> MFYIDNDSGVTVMPPVSAQRSAIVRWFSEGDGNNVITWPGMDWFNIVQAELLNTLEEAGIQPDKTKLNQLALSIKAIMSNNALLIKNNLSEIKTAGASAQRTARENLDIYDASLNKKGLVQLTSATDSPSETLAATAKAVKIAMDNANARLAKDRNGADIPNKPLFIQNLGLQETVNRARNAVQKNGDTLSGGLTFENDSILAWIRNTDWAKIGFKNDADSDTDSYMWFETGDNGNEYFKWRSKQSTTTKDLMNLKWDALSVLVNAIVNGEVISKSANGLRIAYGNYGFFIRNDGSNTYFMLTNSGDNMGTYNGLRPLWINNATGAVSMGRGLNVSGDTLSDRFAINSSNGMWIQMRDNNAIFGKNIVNTDSAQALLRQNHADRKFMIGGLGNKQFGIYMINNSRTANGTDGQAYMDNNGNWLCG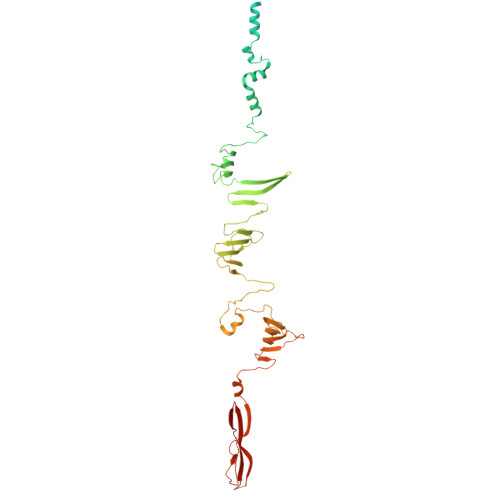AQVIPGNYANFDSRYVRDVRLGTQSLTGGLSRDYKAPSGHVITGFHTNGDWEMQGGDDKVYIRPVQKNINGTWYNVASA> KPKLLNKFDKTIKAELDAAEKLRKRGKIEEAVNAFKELVRKYPQSPRARYGKAQCEDDLAEKRRSNEVLRGAIETYQEVASLPDVPADLLKLSLKRRSDRQQFLGHMRGSLLTLQRLVQLFPNDTSLKNDLGVGYLLIGDNDNAKKVYEEVLSVTPNDGFAKVHYGFILKAQNKIAESIPYLKEGIESGDPGTDDGRFYFHLGDAMQRVGNKEAYKWYELGHKRGHFASVWQRSLYNVNGLKAQPWWTPKETGYTELVKSLERNWKLIRDEGLAVMDKAKGLFLPEDENLREKGDWSQFTLWQQGRRNENACKGAPKTCTLLEKFPETTGCRRGQIKYSIMHPGTHVWPHTGPTNCRLRMHLGLVIPKEGCKIRCANETKTWEEGKVLIFDDSFEHEVWQDASSFRLIFIVDVWHPELTPQQRRSLPAI;> DGDQSETSPSQNQGKCKDGLGEYTCTSLEGFEGKNSELF

Aspartate/asparagine-β-hydroxylase (AspH) is a human 2OG oxygenase catalyzing post-translational hydroxylation of Asp/Asn-residues in epidermal growth factor-like domains (EGFDs) in the endoplasmic reticulum. The human 2OG oxygenase aspartate/asparagine-β-hydroxylase (AspH, BAH, HAAH)13 is highly unusual amongst human 2OG dependent hydroxylases, because its Fe(ii) cofactor is complexed by only two residues (His679 and His725) rather than by the typical triad of ligands (HXD/E⋯H) found in other human 2OG oxygenases. AspH is of significant interest from a cancer research perspective, because its levels are upregulated in invasive cancers (e.g. hepatocellular carcinoma16 and pancreatic cancer17) and it is translocated to the cell surface where it can be used as a diagnostic and prognostic marker. Thus, the combined crystallographic analyses reveal that the C3/C4-substituted 2OG derivatives bind AspH in the same general manner as 2OG, with near identical binding modes for the oxalyl-groups and the C5-carboxylates.

Evidence for an induced fit substrate binding mechanism involving this conformational change has been described when the cosubstrate 2OG was substituted for NOG. The significant conformational changes in the AspH oxygenase domain triggered by substrate binding (ESI Fig. S10†) do not affect the observed mode of 2OG binding in the active site; the binding modes of both 2OG and NOG are very similar, both in the presence or absence of substrate (ESI Fig. S9†). Whilst the oxalyl-groups of both 2OG and (R)-16 bind the metal in an identical manner and the two C5-carboxylate groups are superimposable, the C3- and C4-methylenes adopt different conformations.> SGRAFGEQLLKNPLIEFCDSVCRGCGQVMFQNNTVTGLLFFAGIFYNSTTLGVCAVLGTAASTLTAQLLGVDKPLVRAGLFGANGTLAGIALPFFFNYEPAMLGYVALNGAFTTIIMASLLNFLGKWGVPALTAPFVLATWLLMFGVYKLSLFHPGALIAPALPSVAGLADMGTVTGRTFMEGLFKGVGEVMFQDNIVTGVIFVVAILVNSRISALFAVIGSLVGLCTALIMHSPETPVRLGLYGFNSVLCGIAMGGIFFYLNIRTFLYALGCMVLGAIATGAFSVLLSPIGMPALTWPFIVVTWLFLFAGSMFRNIAQVPTEKAGTPEDNLR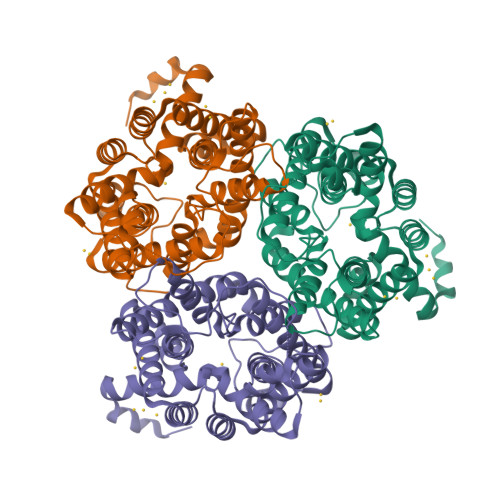SLAIGSR>GDNPCAAGPPVDTNPAECCPKPMLVDGTIMMDCYKKYGEQTKKQLQMDGIPRGCCIAECAMNATNMYADGMLKRDDLSKMFMDAVKDKPEWMSLVRDATNACFELAEKKMDEIEAGAKLEPSFEGEKICHPISGTILRCMGMMMFAQ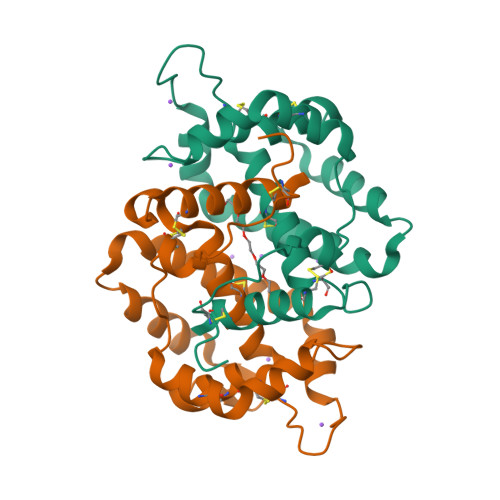CPASVFNVNENCNKLREYGSICPMI[2x]>MDERDALRISREIAGEVRKAIASMPLRERVKDVGMGKDGTPTKAADRVAEDAALEILRKERVTVVTEESGVLGEGDVFVALDPLD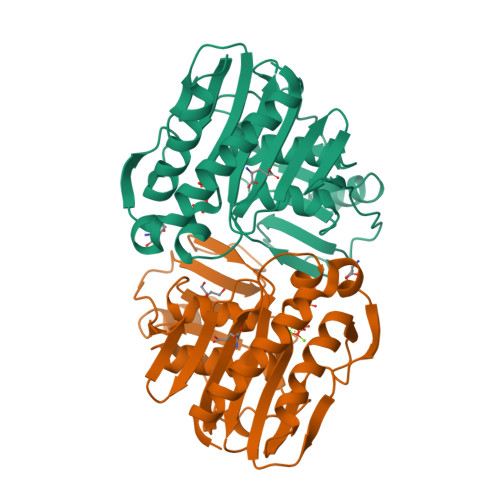GTFNATRGIPVYSVSLCFSYSDKLKDAFFGYVYNLATGDEYYADSSGAYRNGERIEVSDAEELYCNAIIYYPDRKFPFKRMRIFGSAATELCFFADGSFDCFLDIRPGKMLRIYDAAAGVFIAEKAGGKVTELDGESLGNKKFDMQERLNIVAANEKLHPKLLELIK[2x]>[8x]GDPVTTGKPNILIIMVDQLNGKLFPDGPADFLHAPNLKALAKRSARFHNNYTSSPLCAPARASFMAGQLPSRTRVYDNAAEYQSSIPTYAHHLRRAGYYTALSGKMHFVGPDQLHGFEERLTTDIYPADFGWTPDYRKPGERIDWWYHNLGSVTGAGVAEITNQMEYDDEVAFLANQKLYQLSRENDDESRRPWCLTVSFTHPHDPYVARRKFWDLYEDCEHLTPEVGAIPLDEQDPHSQRIMLSCDYQNFDVTEENVRRSRRAYFANISYLDEKVGELIDTLTRTRMLDDTLILFCSDHGDMLGERGLWFK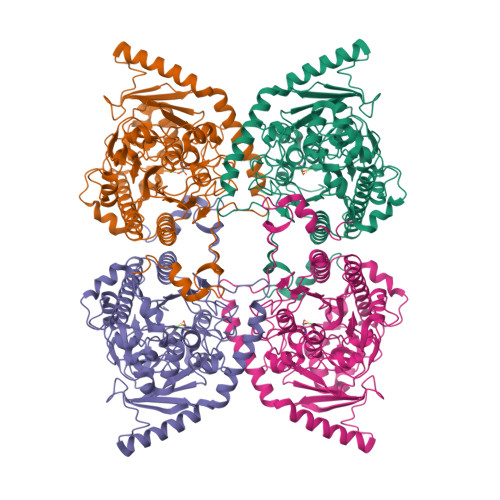MNFFEGSARVPLMIAGPGIAPGLHLTPTSNLDVTPTLADLAGISLEEVRPWTDGVSLVPMVNGVERTEPVLMEYAAEASYAPLVAIREGKWKYVYCALDPEQLFDLEADPLELTNLAENPRGPVDQATLTAFRDMRAAHWDMEAFDAAVRESQARRWVVYEALRNGAYYPWDHQPLQKASERYMRNHMNLDTLEESKRYPRGE For example, unfractionated saliva from Rhipicephalus sanguineus inhibits dendritic cell maturation and differentiation; Salp15, an Ixodes scapularis salivary gland protein, inhibits dendritic cell secretion of pro-inflammatory cytokines; while Japanin, an 18 kDa protein recently isolated from the salivary glands of a hard tick, Rhipicephalus appendiculatus (the Brown Ear Tick), works through currently undefined mechanisms to block DC differentiation from monocytes and inhibits upregulation of co-stimulatory molecules and pro-inflammatory cytokines in response to stimuli. Japanin is predicted from sequence data to be a lipocalin, a member of a family of ubiquitous small proteins found in both prokaryotes and eukaryotes. To provide insight into Japanin’s mechanism of action, we here present two crystal structures of the protein. They reveal that Japanin exists in complex with cholesterol and that it forms a dimer, as well as confirming the prediction from primary sequence that it adopts the lipocalin fold. As was predicted from the sequence, the protein folds as a lipocalin, with an 8-stranded anti-parallel barrel at its centre.

We obtained two crystal structures of recombinantly expressed R. appendiculatus Japanin: (i) a tetragonal form with one copy per asymmetric unit (data to 2.2 Å) and (ii) an orthorhombic one with two molecules per asymmetric unit (data to 2.4 Å), both in complex with cholesterol. In the orthorhombic form, the two molecules in the asymmetric unit form the dimer. The dimer interface involves the 67–75 and 105–112 loops, the 93–99 strand and the 129–141 helix. Figure 2b shows details of the dimer interface between molecules A and B in the lattice, centred around the Phe93A:Phe93B side chain stacking contact, with two additional pairs of hydrophobic residues forming contacts across the interface: Pro139A:Tyr70B and Tyr97A:Ile137B (and equivalent ones due to the twofold symmetry of the dimer, Pro139B:Tyr70A and Tyr97B:Ile137A). Buried in the middle of this hydrophobic patch are the 2.0 Å hydrogen bonds between the side chain of Arg95 on one molecule and the main chain oxygen atom of Ile 94 on the neighbouring molecule. At the surface rim of the interface the Asp98A:Arg132B (and Arg132A:Asp98B) salt bridges are found. In the tetragonal crystals, the same dimer is formed by the asymmetric unit and a symmetry-related molecule across a twofold axis. The tetragonal crystal-form dimer and the orthorhombic crystal-form dimer superpose with an rmsd of 1.5 Å over 297 Cαs. The dimer is likely to represent the solution species, as indicated by Multi-Angle Laser Light Scattering (MALLS) in solution. All three crystallographically-independent molecules show the same overall structure, and each molecule in the crystals binds one molecule of cholesterol.

>[2x]TPSMPAINTQTLYLAGHSSKLFERNVGCVKTRYLNQTGDWVTRSLIYVFTFDTEPWVTQAGAFQVKWEPYSPLLRVKASDYVRDNLGAKPDYFIRTYDNDFLLLSDLKEVRSTCSLWVTLKYVDRIPETINRTFYTICPDPVPVPFDERCYPGGHHHHHH5'-S-ethyl-5'-thioadenosine | C12 H17 N5 O3 S | 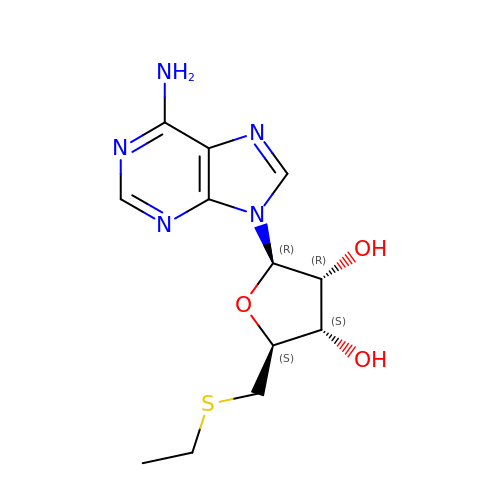HMXHURAGFHWODC-WOUKDFQISA-N>[4x]MEAGITGTWYNQLGSTFIVTAGADGALTGTYVTARGNAESRYVLTGRYDSA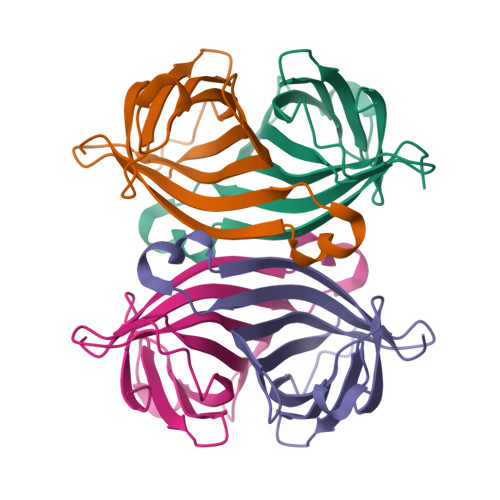PATDGSGTALGWTVAWKNNYRNAHSATTWSGQYVGGAEARINTQWLLTSGTTEANAWKSTLVGHDTFTKVKPSAAS> GAEFKGLRRHMFLYNLTLQRATGISFAIHGNFSGTKQQEIVVSRGKILELLRPDPNTGKVHTLLTVEVFGVIRSLMAFRLTGGTKDYIVVGSDSGRIVILEYQPSKNMFEKIHQETFGKSGCRRIVPGQFLAVDPKGRAVMISAIEKQKLVYILNRDAAARLTISSPLEAHKANTLVYHVVGVDVGFENPMFACLEMDYEEADNDPTGEAAANTQQTLTFYELDLGLNHVVRKYSEPLEEHGNFLITVPGGSDGPSGVLICSENYITYKNFGDQPDIRCPIPRRRNDLDDPERGMIFVCSATHKTKSMFFFLAQTEQGDIFKITLETDEDMVTEIRLKYFDTVPVAAAMCVLKTGFLFVASEFGNHYLYQIAHLGDDDEEPEFSSAMPLEEGDTFFFQPRPLKNLVLVDELDSLSPILFCQIADLANEDTPQLYVACGRGPRSSLRVLRHGLGGNGNSGEKLGAVFNQVAFPLQYTPRKFVIHPESNNLIIIETDHNAYTEATKAQRKQQMAEEMVEAAGEDERELAAEMAAAFLNENLPESIFGAPKAGNGQWASVIRVMNPIQGNTLDLVQLEQNEAAFSVAVCRFSNTGEDWYVLVGVAKDLILNPRSVAGGFVYTYKLVNNGEKLEFLHKTPVEEVPAAIAPFQGRVLIGVGKLLRVYDLGKKKLLRKCENKHIANYISGIQTIGHRVIVSDVQESFIWVRYKRNENQLIIFADDTYPRWVTTASLLDYDTVAGADKFGNICVVRLPPNTNDEVDSQKAEVIMNYHVGETVLSLQKTTLIPGGSESLVYTTLSGGIGILVPFTSHEDHDFFQHVEMHLRSEHPPLCGRDHLSFRSYYFPVKNVIDGDLCEQFNSMEPNKQKNVSEELDRTPPEVSKKLEDIRTRYAQLEQNEAAF;> MTDRYTIHSQLEHLQSKYIGTGHADTTKWEWLVNQHRDSYCSYMGHFDLLNYFAIAENESKARVRFN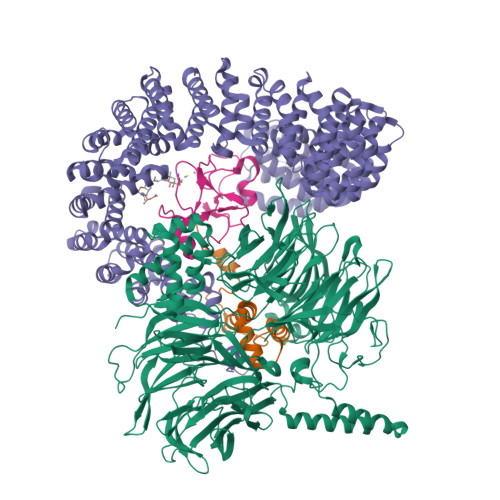LMEKMLQPCGPPADKPEEN;> MKSVNDQPSGNLPFLKPDDIQYFDKLLVDVDESTLSPEEQKERKIMKLLLKIKNGTPPMRKAALRQITDKAREFGAGPLFNQILPLLMSPTLEDQERHLLVKVIDRILYKLDDLVRPYVHKILVVIEPLLIDEDYYARVEGREIISNLAKAAGLATMISTMRPDIDNMDEYVRNTTARAFAVVASALGIPSLLPFLKAVCKSKKSWQARHTGIKIVQQIAILMGCAILPHLRSLVEIIEHGLVDEQQKVRTISALAIAALAEAATPYGIESFDSVLKPLWKGIRQHRGKGLAAFLKAIGYLIPLMDAEYANYYTREVMLILIREFQSPDEEMKKIVLKVVKQCCGTDGVEANYIKTEILPPFFKHFWQHRMALDRRNYRQLVDTTVELANKVGAAEIISRIVDDLKDEAEQYRKMVMETIEKIMGNLGAADIDHKLEEQLIDGILYAFQEQTTEDSVMLNGFGTVVNALGKRVKPYLPQICGTVLWRLNNKSAKVRQQAADLISRTAVVMKTCQEEKLMGHLGVVLYEYLGEEYPEVLGSILGALKAIVNVIGMHKMTPPIKDLLPRLTPILKNRHEKVQENCIDLVGRIADRGAEYVSAREWMRICFELLELLKAHKKAIRRATVNTFGYIAKAIGPHDVLATLLNNLKVQERQNRVCTTVAIAIVAETCSPFTVLPALMNEYRVPELNVQNGVLKSLSFLFEYIGEMGKDYIYAVTPLLEDALMDRDLVHRQTASAVVQHMSLGVYGFGCEDSLNHLLNYVWPNVFETSPHVIQAVMGALEGLRVAIGPCRMLQYCLQGLFHPARKVRDVYWKIYNSIYIGSQDALIAHYPRIYNDDKNTYIRYELDYIL;> GPLGSPGSRAMAKHHPDLIFCRKQAGVAIGRLCEKCDGKCVICDSYVRPCTLVRICDECNYGSYQGRCVICGGPGVSDAYYCKECTIQEKDRDGCPKIVNLGSSKTDL>[2x]HMAKHQIGVIG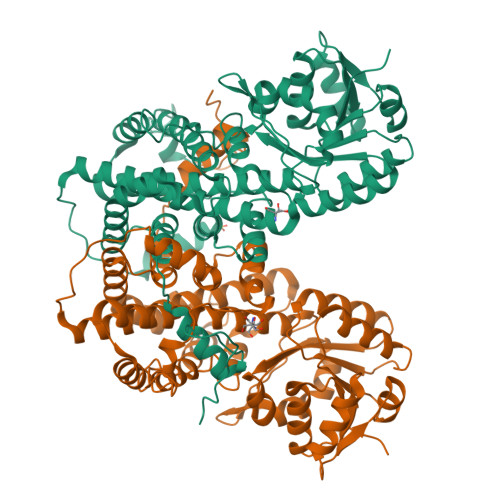LAVMGKNLALNIESKGYSVAVYNRLREKTDEFLQEAKGKNIVGTYSIEEFVNALEKPRKILLMVKAGAPTDATIEQLKPHLEKGDIVIDGGNTYFKDTQRRNKELAELGIHFIGTGVSGGEEGALKGPSIMPGGQKEAHELVRPIFEAIAAKVDGEPCTTYIGPDGAGHYVKMVHNGIEYGDMQLIAEAYFLLKHVLGMDAAELHEVFADWNKGELNSYLIEITADIFTKIDEETGKPLVDVILDKAGQKGTGKWTSQNALDLGVPLPIITESVFARFLSAMKDERVKASKVLAGPAVKPFEGDRAHFIEAVRRALYMSKICSYAQGFAQMKAASEEYNWNLRYGDIAMIFRGGCIIRAQFLQKIKEAYDRDPALSNLLLDSYFKDIVERYQDALREIVATAAMRGIPVPGSASALAYYDSYRTAVLPANLIQAQRDYFGAHTYERVDKEGIFHTEWLK> SMEKEIKKWSVYFQNPEFLERTRMFLIQKELYPLVRNWCGVKDNVRLLDVGCGTGYFTRLLVSGDEDVSAVGIDMEEPFIEYAREK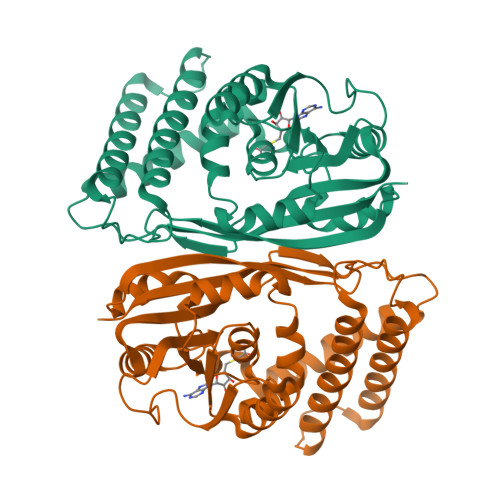AEELGLPAEFIIGDALALPFEDNTFDIVTSHTFLTSVPDPEKAMSEMKRVVKPGGIISSVTAMNFMPACNNEGEYPEECTWVEDLKKEYMKIYTKYFSADPLETRIKGVKCSDVPKFFTGQGLKDVSLYPIGKVFTLSNAAVSDEDKLRYIELFYASEIKKLDAFMELPDEDIGITEEDAERFRSLIGQKCKWLRDHLHDNYAWEWQGGANLLVTGICNKQR>MDTNPCEKHSCIAVIDAGSTGSRLHIYSYDTDDTNTPIHIEEIWNKKIKPGFASIQPNSVTIDAYLTMLLADAPIHNIPVYFYATAGMRLLPQSQQKKYYDELDYWFRQQSQWQLVEAK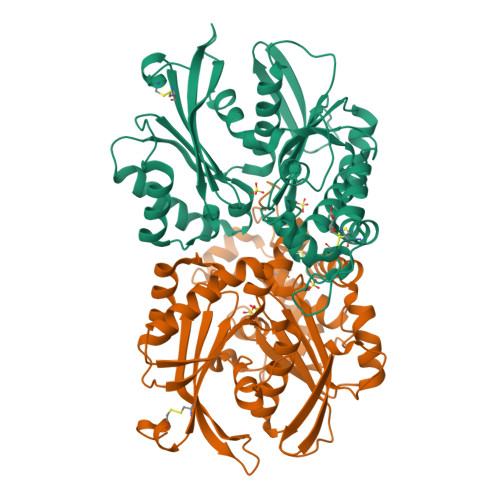TITGNDEALFDWLAVNYKLDTLKSVQNKSVGVMDMGGASVQIVFPMPKNAEISKHNQVELNIYGQNINLYVHSFLGLGQTEMSHQFLNSPSCFANDYPLPDGESGQGNAPSCKEEVTSLMNSVHKVNQQIQPLLALNPVNEWYSIGGISNLASSQLFHFENSELTNQSLLQQGDNQICHQQWDILNGQYPDDEYLYQYCLLSSYYYALMVDGYGINPNQTIHYIPPEQNLDWTIGVVLHRALEHHHHHH[2x]> GPLGSEDDLYRQSLEIISRYLREQATGAKDTKPMGRSGATSRKALETLRRVGDGVQRNHETAFQGMLRKLDIKNEGDVKSFSRVMVHVFKDGVTNWGRIVTLISFGAFVAKHLKSVNQESFIEPLAETITDVLV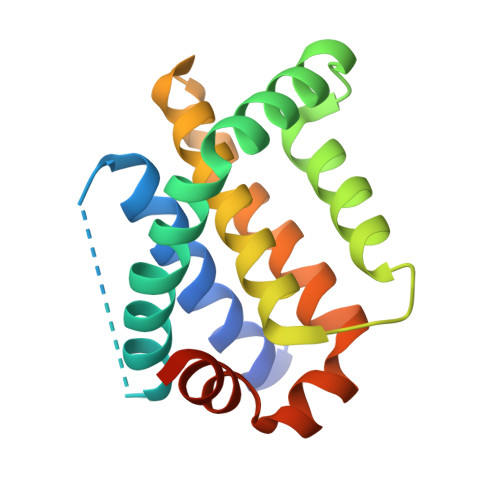RTKRDWLVKQRGWDGFVEFFHVQDLEGG>MSMIETWTAVDQYVSDVLIPKDSTLEEVLQVNAAANLPAHDVSPTQGKFLQLLVQIQGARNILEIGTLGGYSTIWLARGLSSGGRVVTLEASEKHADIARSNIERANLNDRVEVRTGLALDSLQQIENEKYEPFDFIFIDADKQNNPAYFEWAL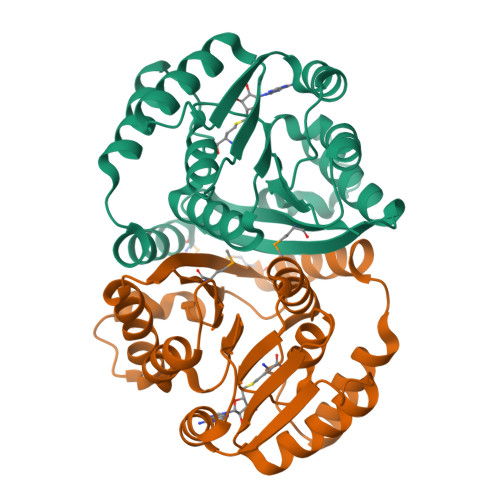KLSRPGTVIIGDNVVREGEVIDNTSNDPRVQGIRRFYELIAAEPRVSATALQTVGSKGYDGFIMAVVKE[2x]ANTAR domains are a class of antiterminator that bind and stabilize dual hexaloop RNA motifs within the nascent RNA chain to prevent terminator loop formation. EutV possesses one of the most common domains architectures found among all ANTAR proteins annotated in the Pfam database, consisting of an N-terminal phosphor-sensitive REC domain (aa 1–119) coupled to a C-terminal ANTAR domain (aa 141–186) via a coiled-coil domain. Ethanolamine (EA) stimulates the histidine kinase EutW (component 1) to phosphorylate EutV (component 2) which promotes homodimerization of the protein. Dimeric EutV acts as an antiterminator of RNAP by binding these dual hexaloop motifs within the nascent mRNA chain inhibiting T-loop formation and thereby preventing transcription termination.

Additional density present at Asp 54 on both chains indicated successful incorporation of BeF3– and activation of EutV. Unambiguous electron density for a single RNA hexaloop was present at the ANTAR domain of each EutV chain. The dual hexaloop RNA molecule was bridging between two asymmetric units within the crystal lattice with each hexaloop contacting a symmetry-related ANTAR domain of EutV in the neighbouring ASUs. In total, each ASU contains an asymmetric dimer of EutV and two RNA hexaloops from different RNA molecules. As a result, chain a and b make more interactions with the P2 RNA hexaloop than P1. Both sites bind a single hexaloop with the conserved G4 of each loop flipping outward to form π–π stacking interactions with Tyr164 of the ANTAR domain. The G4 of P2 is coordinated by hydrogen bonds to Arg142, Lys149 and Glu160 of chain b, however, Arg142 from chain a is unable to make the same contact with P1 (compare A and C). Intriguingly, residues Lys143 and Lys147 from chain a contact the P2 RNA, through hydrogen bonds to the phosphate and ribose respectively, representing the only interactions between an ANTAR domain and the RNA hexaloop located on the opposite protein chain. Asn173 and Arg175 hydrogen bond with hydroxyl groups of the ribose sugars of the bases that form the stem of the hexaloop, and Arg177 makes a hydrogen bond to the phosphate backbone of the base at position 2 of the hexaloop. Unexpectedly, given its hydrophobic nature, Met172 is positioned in the middle of the hexaloop of the RNA hairpin and may act as a hydrophobic plug to position the hexaloop on α7 within the ANTAR domain and flip the G4 base out of the hexaloop. Nevertheless, there is a break in symmetry of the homodimer upon RNA binding due to a larger flex in the coiled-coil of chain b, between Ile139-Glu141, than for chain a.

>SNMDGRIVIVDDEPITRLDIRDIVIEAGYEVVGEAADGFEAIEVCKKTQPDLVLMDIQMPILDGLKAGKKIVQDQLASSIVFLSAYSDVQNTDKAKKLGALGYLVKPLDEKSLIPTIEMSIERGKQTQLLLSQIDKLSLKLEERKIIEKAKGILVKENHISEEEAYQMLRTLSMNKRARMSEIAELIVMDDE[2x]In the human pathogen Staphylococcus aureus, c-di-AMP is produced by the di-adenylate cyclase enzyme DacA, which is thought to form a complex and be regulated by YbbR and GlmM, two other conserved proteins. GlmM codes for the essential phosphoglucosamine mutase enzyme, required for the conversion of glucosamine-6-phosphate to the early peptidoglycan synthesis precursor glucosamine-1-phosphate. We determined the atomic structures of the S. aureus DacA and GlmM enzymes and show that GlmM readily binds to DacA in vitro and blocks its activity by masking its active site. Specifically, our data suggest that GlmM blocks access to the active site of DacA and in this manner prevents the formation of catalytically active head-to-head DacA oligomers.

To gain further insight into the function and catalytic mechanism of the S. aureus c-di-AMP cyclase DacA, the soluble catalytic domain starting from amino acid F101 (hereafter referred to as DacACD) was expressed and purified as N-terminal His-tag fusion protein. The S. aureus DacACD protein displayed the expected globular fold, with a central β-sheet made up of 7 antiparallel strands flanked by 5 helices (left). While the L. monocytogenes CdaACD protein was found to be a tetramer in the asymmetric unit (although dimeric in solution), the S. aureus DacACD was present as a symmetric dimer, with two protomers interacting via the backbone of α3, β2 and the loop connecting α3 and β3. At the interface, residue N166 from one protomer formed a hydrogen bond interaction with residue T172 from the second protomer and a van der Waals interaction was formed between residue P173 and residues N166 and I165 of the neighbouring protomer. Further analysis using the PdbePISA program revealed a total buried surface area of 1450 Å2 at the dimer interface with a ΔG (int) of -8.3 kcal/mol and a ΔG (diss) of 2.1 kcal/mol, indicative of a strong protein/protein interaction. In order to condense two ATP molecules to c-di-AMP, two protomers need to be arranged in a head-to-head conformation. However, in the S. aureus DacACD dimer found in the crystallographic asymmetric unit, the active sites of the protomers are outward facing and hence are too far apart for c-di-AMP synthesis. In addition, analysis of the crystal lattice did not reveal any symmetry-related molecule arranged with the catalytic sites in a head-to-head orientation. Here, we show that the S. aureus DacACD protein is a dimer. However, based on the data presented in this study, we suggest that this dimer is not the active unit per se, as the protomers are not found in a head-to-head conformation.

>[2x]GSHMASFLKRYTSNTYSKDEEKLIQSVSKAVQYMAKRRIGALIVFEKETGLQDYIETGIAMDSNISQELLINVFIPNTPLHDGAMIIQGTKIAAAASYLPLSDSPKISKSLGTRHRAAVGISEVSDAFTVIVSEETGDISVTFDGKLRRDISNEIFEELLAEHWFGTRFQKKGVK N,N,N-TRIMETHYL-4-OXOPENTAN-1-AMINIUM | 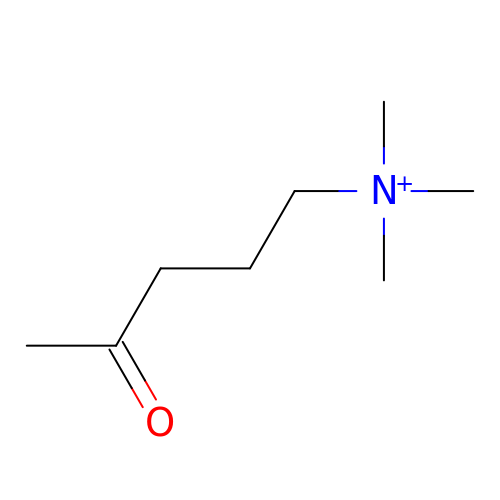C8 H18 N O | UKCYTFTWLWVZSO-UHFFFAOYSA-N> MAQDALSDGFVR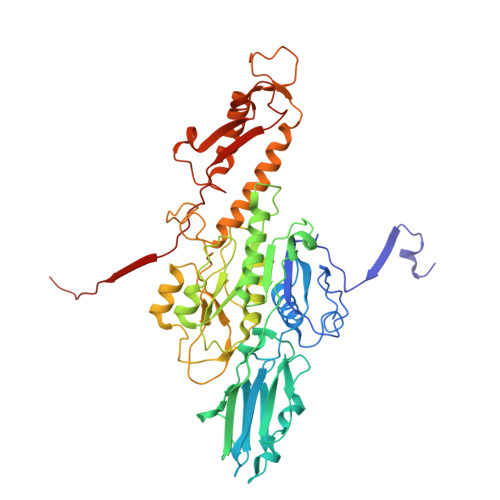LCIDPSLNFFGEGCKILVEGQITDDATAAENVVTCVNSELDLVERFGQGSVLTESLRKVFCMCKSGVSVYALPRADAAAAVSAVYTLTVTGTALTDGRVQLYMGEAEYSLDIGVDEGDTPTQIAAKIVAAISPDFPYEATAAAGVITLTARNGGTIGNHLSVIYTNLGSCTSVTPEGVTVAFAQTTPGSVNPEPNDYASVVNECCFAVYVLSSDDTDWQENLRDWIRSAWDCSKPQCFGHGYVFNKGTLGQVLADGDNSAELSRLALPTTYPVLPYLTNAAYGALSACSTCENPELNVQGQTYGLLSCINMPESCTPGWEFTEVTQLQNNGFVVSGPATTSGQGNFTSPYIYNDVTNYLRDEKNRPNATFRDASSRRLAAATGVALATFLQQFNGLAVFTKNTNIKTGIIGTNLRLMLGKIRKWASDNVGVLFSEFDNINEDIQLVSDFDVQPKCVGQPGVFHLNMRYRPPVRGARINVNLVPALFDNCDR> GSHMEGAGAGSGFRKELVSRLLHLHFKDDKTKVSGDALQL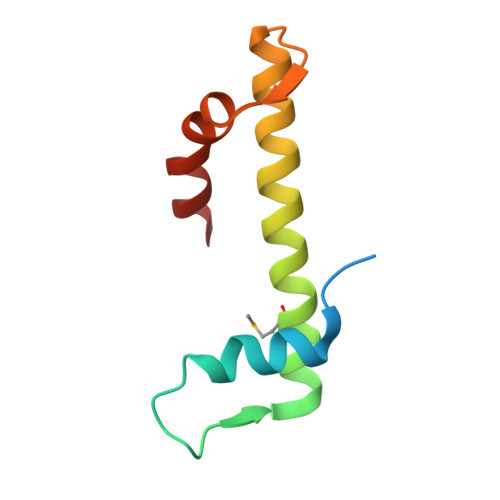MVELLKVFVVEAAVRGVRQAQAEDALRVDVDQLEKVLPQLLLDF> MQTLKELIASNPDDLTTELKRAFRPLTPHIAIDGNELDALTILVNLTDKTDDQKDLLDRAKCKQKLRDEKWWASCINCVNYRQSHNPKFPDIRSEGVIRTQALGELPSFLLSSSKIPPYHWSYSHDSKYVNKSAFLTNEFCWDGEISCLGELLKDADHPLWNTLKKLGCSQKTCKAMAKQLADITLTTINVTLAPNYLTQISLPDSDTSYISLSPVASLSMQSHFHQRLQDENRHSAITRFSRTTNMGVTAMTCGGAFRMLKSGAKFSSPPHHRLNSKRSWLTSEHVQSLKQYQRLNKSLIPENSRIALRRKYKIELQNMVRSWFAMQDHTLDSNILIQHLNHDLSYLGATKRFAYDPAMTKLFTELLKRELSNSINNGEQHTNGSFLVLPNIRVCGATALSSPVTVGIPSLTAFFGFVHAFERNINRTTSSFRVESFAICVHQLHVEKRGLTAEFVEKGDGTISAPATRDDWQCDVVFSLILNTNFAQHIDQDTLVTSLPKRLARGSAKIAIDDFKHINSFSTLETAIESLPIEAGRWLSLYAQSNNNLSDLLAAMTEDHQLMASCVGYHLLEEPKDKPNSLRGYKHAIAECIIGLINSITFSSETDPNTIFWSLKNYQNYLVVQPRSINDETTDKSSL;>MKLPTNLAYERSIDPSDVCFFVVWPDDRKTPLTYNSRTLLGQMEAASLAYDVSGQPIKSATAEALAQGNPHQVDFCHVPYGASHIECSFSVSFSSELRQPYKCNSSKVKQTLVQLVELYETKIGWTELATRYLMNICNGKWLWKNTRKAYCWNIVLTPWPWNGEKVGFEDIRTNYTSRQDFKNNKNWSAIVEMIKTAFSSTDGLAIFEVRATLHLPTNAMVRPSQVFTEKESGSKSKSKTQNSRVFQSTTIDGERSPILGAFKTGAAIATIDDWYPEATEPLRVGRFGVHREDVTCYRHPSTGKDFFSILQQAEHYIEVLSANKTPAQETINDMHFLMANLIKGGMFQHKGD[6x];> MKWYYKTITFLPELCNNESLAAKCLRVLHGFNYQYETRNIGVSFPLWCDATVGKKISFVSKNKIELDLLLKQHYFVQMEQLQYFHISNTVLVPEDCTYVSFRRCQSIDKLTAAGLARKIRRLEKRALSRGEQFDPSSFAQKEHTAIAHYHSLGESSKQTNRNFRLNIRMLSEQPREGNSIFSSYGLSNSENSFQPVPLI;>MFLQRPKPYSDESLESFFIRVANKNGYGDVHRFLEATKRFLQDIDHNGYQTFPTDITRINPYSAKNSSSARTAS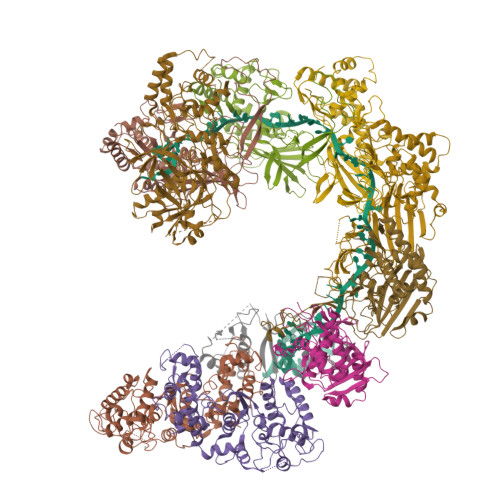FLKLAQLTFNEPPELLGLAINRTNMKYSPSTSAVVRGAEVFPRSLLRTHSIPCCPLCLRENGYASYLWHFQGYEYCHSHNVPLITTCSCGKEFDYRVSGLKGICCKCKEPITLTSRENGHEAACTVSNWLAGHESKPLPNLPKSYRWGLVHWWMGIKDSEFDHFSFVQFFSNWPRSFHSIIEDEVEFNLEHAVVSTSELRLKDLLGRLFFGSIRLPERNLQHNIILGELLCYLENRLWQDKGLIANLKMNALEATVMLNCSLDQIASMVEQRILKPNRKSKPNSPLDVTDYLFHFGDIFCLWLAEFQSDEFNRSFYVSRW[2x]>MNVSIEEFTHFDFQLVPEPSPLDLVITEPLKNHIEVNGVKSGALLPLPFQTGIGKTYTALNFLLQQMLEQVRSELKEENTGKKSKRLLYYVTDSVDNVVSAKADLLKLIEKQTVKGEPRFTLEQQEYLKAQIVHLPNQSEQLLQCSDAVLNDVLIGFNLNAERDVQAEWSAISGLRRHASNPEVKISLNRQAGYFYRNLIDRLQKKQKGADRVLLSGSLLASVETLLPGEKIRNGSAHVAFLTTSKFLKGFHNTRSRYSPLRDLSGAVLIIDEIDKQNQVILSELCKQQAQDLIWAIRTLRANFRDHQLESSPRYDKIEDLFEPLRERLEEFGTNWNLAFAFNTEGANLNERPVRLFSDRSFTHVSSATHKLSLKSDFLRRKNLIFSDEKVEGSLIEKHGLLTRFVNEADVIYQWFLGTMRKAVFQYWENVRGLEIEVRENRSLEGTFQEAVQSLLTHFNLQEFESAVYESFDTRGLRQSAGGKANKLSSSKSYHHTGLKLVEVAHNQGTRDTVNCKASFLNTSPSGVLADMVDAGAVILGISATARADTVIHNFDFKYLNERLGNKLLSLSREQKQRVNNYYHSRRNYKDNGVVLTVKYLNSRDAFLDALLEEYKPEARSSHFILNHYLGIAESEQAFVRSWLSKLLASIKAFISSPDNRYMLSLLNRTLDTTRQNINDFIQFCCDKWAKEFNVKTKTFFGVNADWMRLVGYDEISKHLNTELGKVVVFSTYASMGAGKNPDYAVNLALEGESLISVADVTYSTQLRSDIDSIYLEKPTQLLLSDDYSHTANQLCQFHQILSLQENGELSPKSAENWCRQQLMGMSRERSLQQYHQTSDYQSAVRKYIEQAVGRAGRTSLKRKQILLFVDSGLKEILAEESRDPSLFSHEYVALVNKAKSAGKSIVEDRAVRRLFNLAQRN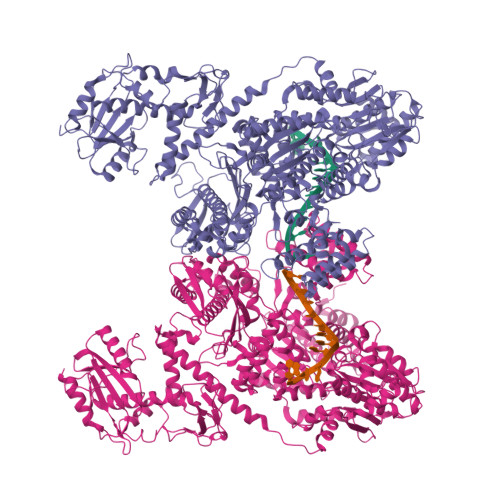NKDGMLSIKALVHRLHNQPASKSDIQEWQDIRTQLLRYPTVAFQPERFNRLYLQSMTKGYYRYQGNLDGDPNSFEFFDRVPYGDMVSEEDCSLATLVQNQYVRPWFERKGFACSWQKEANVMTPIMFTNIYKGALGEQAVEAVLTAFDFTFEEVPNSIYERFDNRVIFAGIEQPIWLDSKYWKHEGNESSEGYSSKIALVEEEFGPSKFIYVNALGDTSKPIRYLNSCFVETSPQLAKVIEIPALIDDSNADTNRTAVQELIKWLHHS[2x]> MTKITVNYTVDVKDIQPKHVRSESNPQNQNKIRRAWVLSLSDNAMEVIQNKIKSAPARHAYYEAIDREVSNKWIELMRKHTTESLNAGAKFIMTSCGERLEDDYCGNADERLIVAAQIVAETI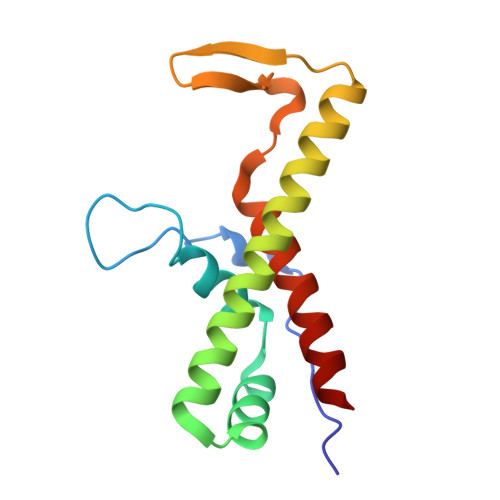AADFNR>SIQVIARAASIMRALGSHPHGLSLAAIAQLVGLPRSTVQRIINALEEEFLVEALGPAGGFRLGPALGQLINQAQTDILSLVKPYLRSLAEELDESVSLASLAGDKIYVLDRIVSERELRVVFPIGINVPAAATAAGKVLLAALPDETLQAALGEQLPVLTSNTLGRKALVKQLSEVRQSGVASDLDEHIDGVSSFATLLDTYLGYYSLAIVMPSSRASKQSDLIKKALLQSKLNIERAIGR[4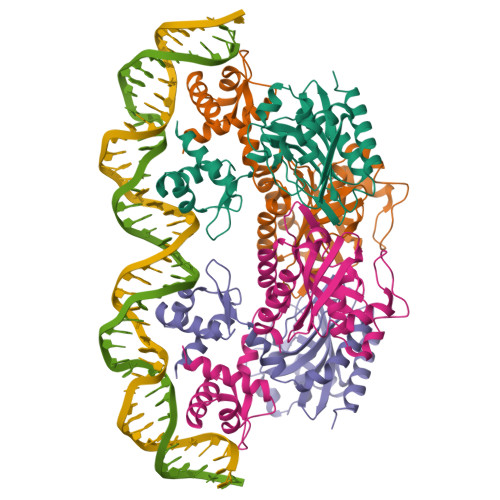x]>MSHIFDASVLAPHIPSNLPDNFKVRPLAKDDFSKGYVDLLSQLTSVGNLDQEAFEKRFEAMRTSVPNYHIVVIEDSNSQKVVASASLVVEMKFIHGAGSRGRVEDVVVDTEMRRQKLGAVLLKTLVSLGKSLGVYKISLECVP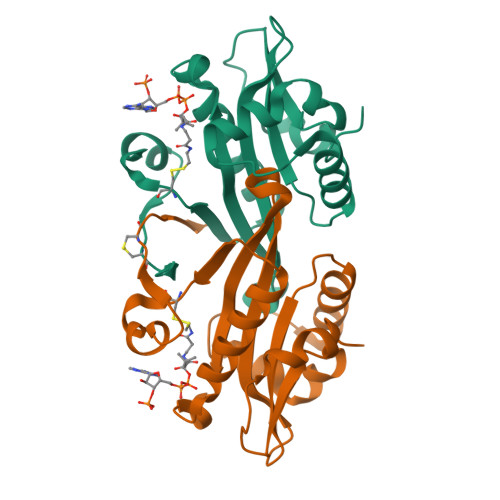ELLPFYSQFGFQDDCNFMTQRF[2x]(4Z)-4-(2-AMINO-5-OXO-3,5-DIHYDRO-4H-IMIDAZOL-4-YLIDENE)-2,3-DICHLORO-4,5,6,7-TETRAHYDROPYRROLO[2,3-C]AZEPIN-8(1H)-ONE | C11 H9 Cl2 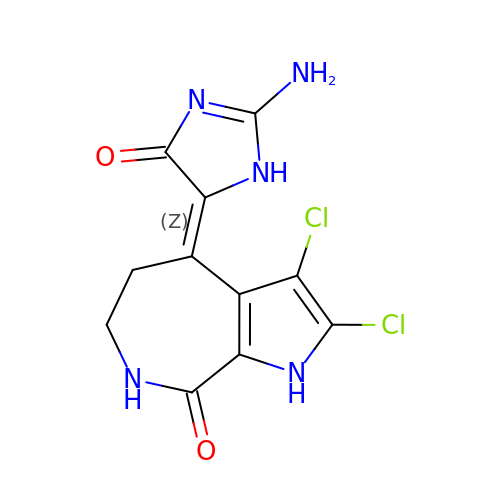N5 O2 | WMIYIBXBFBOKCT-UTCJRWHESA-N>MPWKGISGSLSRISAGSVTNVWGVNAANNIYRYTGDDAKPWVQIPGALTDIGAAADGTVWGVNAAGNIYRYVWDSNHWTQIKGALKRISAGSRTNVWGVNAGGAIYRYTGDDANPWVQIPGVLSDIGAGADGTVWGVNAAGEIYRYTGDQGDPNHWVKIPGALSAISAGIKTNVWGVNSANNIYTSTGDDK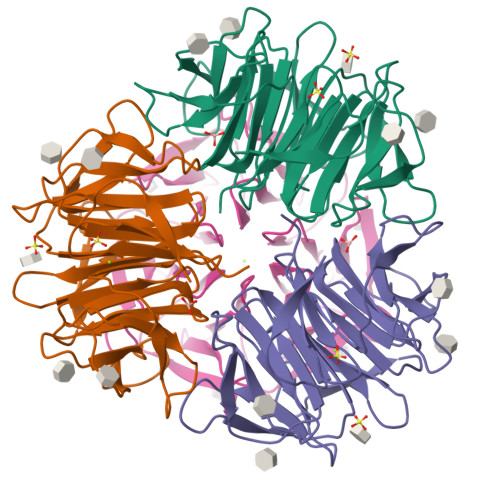NPWLGIGGSLVDIGAGTDGVVWGVNAGGGIYRWIRD[2x]[(2~{R},3~{S},4~{S})-5-[[2,5-bis(azanyl)-6-oxidanylidene-1~{H}-pyrimidin-4-yl]amino]-2,3,4-tris(oxidanyl)pentyl] 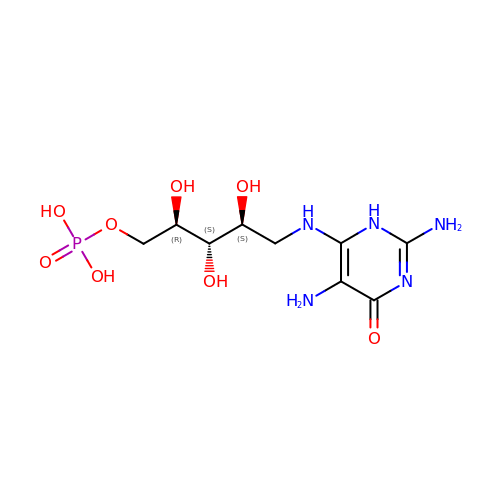dihydrogen phosphate | C9 H18 N5 O8 P | ACIVVGBVOVHFPQ-RPDRRWSUSA-N Here, we identify and characterize a unique GlcN kinase from the soil bacterium Streptacidiphilus jiangxiensis, closely related to Streptomyces spp., the classical antibiotic producers. In contrast, from 20 sugars and 4 aminoglycoside antibiotics tested, SjGlcNK only phosphorylated specifically GlcN and displayed vestigial activity with glucose using ATP as a phosphate donor. Determination of the Michaelis constants (Km) for glucose and GlcN suggested that SjGlcNK is better described as a GlcN kinase (EC 2.7.1.8) with a strong preference for using GlcN (Km = 8 ± 1 mM) over glucose (Km > 100 mM) as the substrate. In addition, the structural and biochemical characterization of SjGlcNK provides new insights into the role of these unique GlcN kinases as the missing link for the incorporation of environmental GlcN to the metabolism of GlcNAc in bacteria, an important intermediate in peptidoglycan biosynthesis, glycolysis, and secondary metabolite production.

SjGlcNK was crystallized in two different monoclinic (P21) crystal forms, A and B, which differ considerably in the dimensions of the respective unit cells. In consequence, there are two SjGlcNK molecules in the asymmetric unit (AU) of crystal form A, while four monomers are found in the larger AU of crystal form B. The individual structures of the N-terminal cap, the intermediate subdomain, and the C-lobe are highly conserved in the six protomers, across the two crystal forms. In contrast to the structural conservation of the individual subdomains, the relative positions of the N- and C-lobes are strikingly different in the six molecules. In result, the distance between equivalent atoms in the N- and C-lobe varies from 31.7 Å in the open to 20.6 Å in the closed conformation, and superposition of the C-lobe (residues 194 to 420) of the six different conformational states results in RMSD values ranging from 0.6 to 5.6 Å for the whole molecule. Principal-component (PC) analysis revealed that the six conformers of SjGlcNK are related by an opening-closure movement (PC1), i.e., a hinge-bending motion of the N- and C-lobes of ∼30° amplitude. In this movement, the linker connecting the two lobes (residues 187 to 191) acts as a hinge and the catalytic lysine, K133, which sits far from the active site in the open state I, approaches and establishes contacts with the catalytic D317 in the closed state VI, likely corresponding to the active conformation of the enzyme. In summary, ATP induces the closure of SjGlcNK, and the crystallographic structures reported represent six different conformational snapshots of the enzyme, arising from the molecular flexibility required to carry out its catalytic cycle. Curiously, the conformation of the side chain of D317 changes between the nucleotide-free (where it is coordinating the single and more tightly bound Mg1) and the quaternary complex structure (where it coordinates the two magnesium ions).

>MTPNWSELVAAADPALVLPSGERRAEVAVPGPLRLDALLDLGEGHAVGVVRSADAARWTVPLVRDGAGGVRRSRPGDGTAEHLVAALARRGATPDAAFVLEAFTGAAPVTGERGIIVDQTNESVIVGECAVVKWAVRLPAEGEPGSPAAQRIAALARGGFTEMPRPWGLLTLAEGAQPVLLASVVAYLPGALDGWDWAVDDVRRLARGELTMDQALLPAAQLGTLTARMHAALAARGRTPATAADVAAWGVRMREELDEAVASVPGAEGERLKAWAPRIADVYAELDALAGTPLIDVHGDFHVGQILRADGRYAVVDFDGNPVLPADQRAARQPAALDVVGMTASLDHVGRVVVFRTPDVDPAPVRAWIAAAQRSFLDAYRTTLARLDADDLFDDRLLTPLRYAQEVREYLYAVRHLPHWVYVPDLSLTDLLPERLKDKLAAALEHHHHHH[4x]> MAISIKTPEDIEKMRVAGRLAAEVLEMIEPYVKPGVSTGELDRICNDYIVNEQHA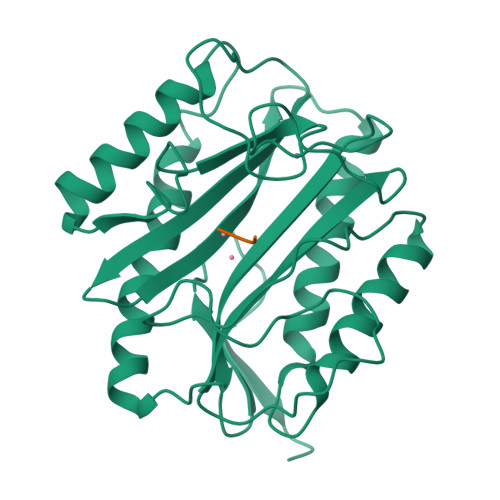VSACLGYHGYPKSVCISINEVVCHGIPDDAKLLKDGDIVNIDVTVIKDGFHGDTSKMFIVGKPTIMGERLCRITQESLYLALRMVKPGINLREIGAAIQKFVEAEGFSVVREYCGHGIGQGFHEEPQVLHYDSRETNVVLKPGMTFTIEPMVNAGKKEIRTMKDGWTVKTKDRSLSAQYEHTIVVTDNGCEILTLRKDDTIPAIISHDEL> MRGSHHHHHHGSMTDITGVCPDRFAAVREVFEQNFADG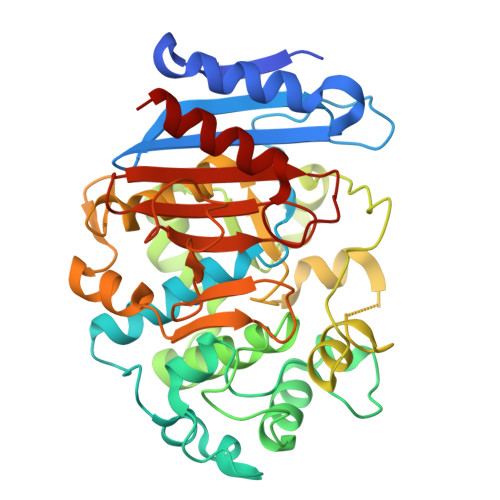GELGARFAFAIEGEVVVDLMGGFADRKRQVPFGPDTLTALFSTTKAVAALLIARLVDEGRLAYDQAVADVWPEFAQAGKDAVTVEQALSHQAGLSGFPDETDPAIWFDWDATCAKLAAMAPLFPIGSASGYHPVTYGYLAGEIFRRVDGRTMGTALREDICEPLGLDLWIGLPDSEHDRVADLMRPTAMPQFGEINPAVEAAFFKPWSSPGGKGAAEWRRVEIPSANGHATAPALARLMGALAHGGTLDGRSLITPAGIKAATAERLRGRDLVLPYEISWGAGFMRNEPNFYYGPTAEAFGHSGWGGSCAFADPTRGVSGAYVMNKQGNALIGDPRSVRLIEAAYASL>LPEQIDWRKKGAVTPVKNQGKCGSCWAFSTVSTVESINQIRTGNLISLSEQQLVDCNKKNHGCKGGAFVYAYQYIIDNGGIDTEANYPYKAVQGPCRAAKKVVRIDGYKGVPHCNENALKKAVASQPSVVAIDASSKQFQHYKSGIFSGPCGTKLNHGVVIVGYWKDYWIVRNSWGR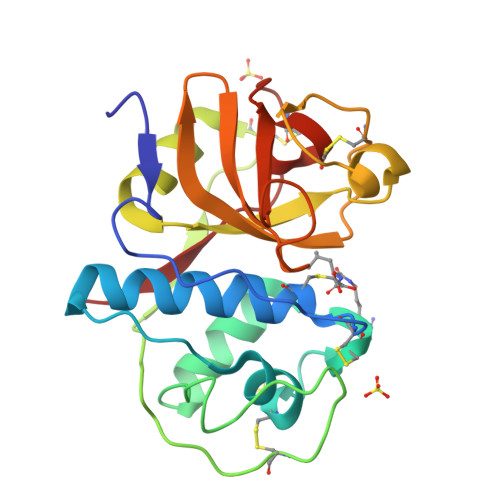YWGEQGYIRMKRVGGCGLCGIARLPYYPTKA[2x]N-{4-[(1S)-1-aminoethyl]phenyl}cyclopropanecarboxamide 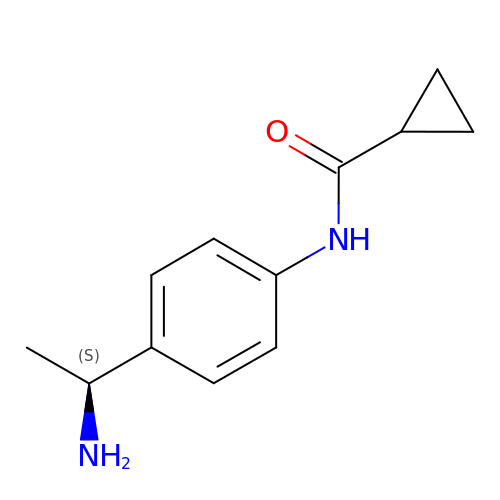| C12 H16 N2 O | CELFORIQAQLUCB-QMMMGPOBSA-N>GMQVEQRTLNTAAHPFQITAYWLDQISDFETAVDYPIMIICPGGGFTYHSGREEAPIATRMMAAGMHTVVLNYQLIVGDQSVYPWALQQLGATIDWITTQASAHHVDCQRIILAGFSAGGHVVATYNGVATQPELRTRYHLDHYQGQHAAIILGYPVIDLTAGFPTTSAARNQITTDARLWAAQRLVTPASKPAFVWQTATDESVPPINSLKYVQAMLQHQVATAYHLFGSGI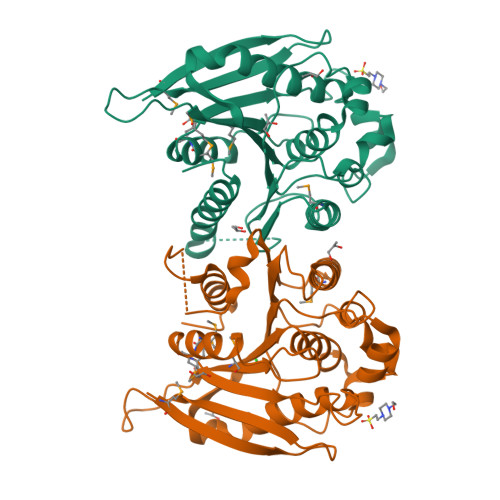HGLALANHVTQKPGKDKYLNDQAAIWPQLALRWLQEQGLLAGNY[2x]N-[(2S)-1-(hydroxyamino)-3-methyl-3-{[(oxetan-3-yl)methyl]sulfonyl}-1-oxobutan-2-yl]-4-(6-hydroxyhexa-1,3-diyn-1-yl)benzamide | C22 H26 N2 O7 S | 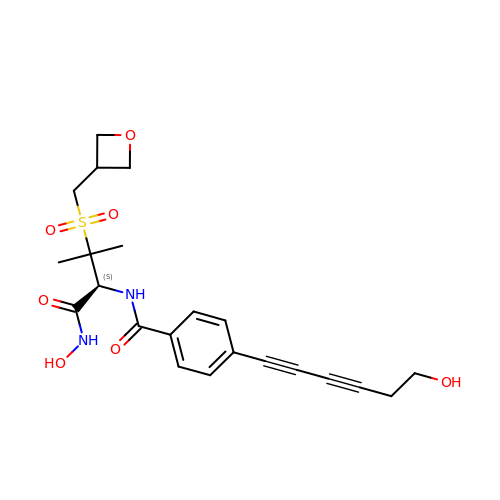HUQFNHQVVJRSBA-IBGZPJMESA-N>[24x]MATEGARNIGQSAPEGKVQMDCPSRHNFDPECEKAFVEHIHLELASSYHAWSMWAFYARDCKAAVGMTRLCEWASHVSAQRARRMAAYVLTRGGHVDYKEIPAPKKQ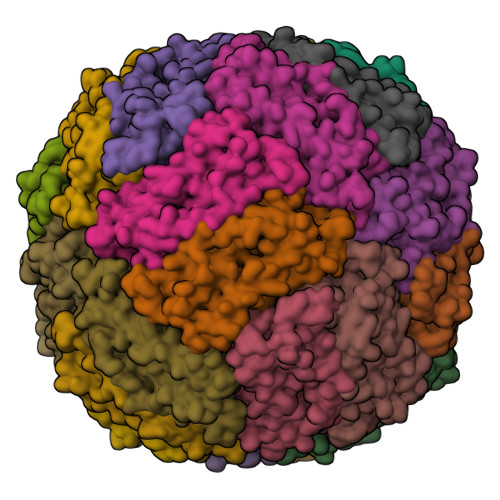GWDNFEDAFSHCVANKKRILTSLQSLYQCCQSKDAHCSNFIQTDMMDEVIAWNKFLSDCLSNLHCIGSQGMGPWVFDRWLARIVMSKFKHPKIPSLSTSDLESNIPNELFDAEGDMVRAIKKL> MLQYTSSARQALRATALVLNFFPLGYTCGPKNKQVFFPPNNLDGRTTHQMKKLQGSTDKHPGLVPRDKLKLHCEFCRFHWVQDTLVVRCAAHPKEHNQREIWLEPTWTWGKQQPYQYYKYMPVNINPRTGMPLAREDAKGM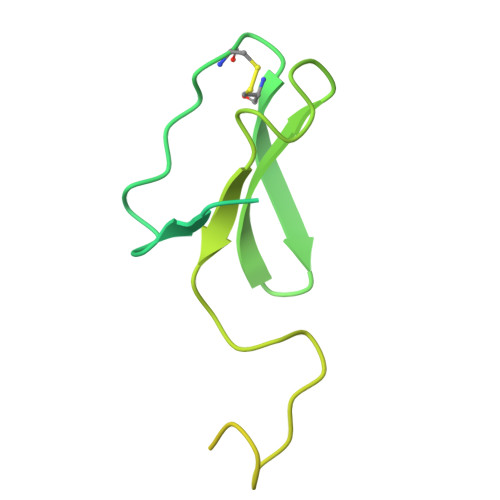NNERRSQGLPTKTRLLERERRGISRAITGLGIYNQRWQTRFPFAT>[6x]MSALPELRELIASFVSEEPPEIRRIRTGTVPDLPGSYGQYFTAWDFSNSIVRDYAMNLYQLTRLATDESVSVENLLTVFRTLDPIYSTFLGYNGFPVLAEYAQRVGQPAESRAELLDRLTTFTEYVNRLTAWSHHYFPWDLGGERYRYAAEEVAAQAAEAAAASPSVDSVDSLGDPSQRIPVRLTWQPLGVQVDAEIYADLNPQLATDVLKALPFTVL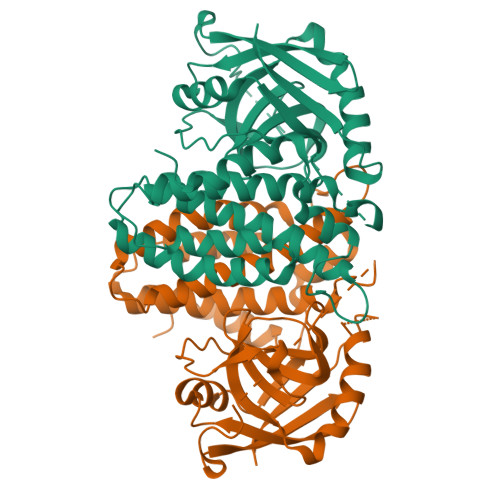QDHAVVSGESMYAWAPLVSVAPTPVRERICDAPVGRLRFSQATGNKVIVQYGPTTETLSSPVLGKVVDSHADRLAEVGKAVWESTFSSKEPVWLTVERL>MILVNKETRVLVQGITGREGQFHTKQMLSYGTKIVAGVTPGKGGMEVLGVPVYDTVKEAVAHHEVDASIIFVPAPAAADAALEAAHAGIPLIVLITEGIPTLDMVRAVEEIKALGSRLIGGNCPGIISAEETKIGIMPGHVFKRGRVGIISRSGTLTYEAAAALSQAGLGTTTTVGIGGDPVIGTTFKDLLPLFNEDPETEAVVLIGEIGGSDEEEAAAWVKDHMKKPVVGFIGGRSAPKGKRMGHAGAIIMGNVGTPESKLRAFAEAGIPVADTIDEIVELVKKALGWNSRPGIL[4x];>[4x]MNLHEYQAKEILARYGVPVPPGKVAYTPEEAKRIAEEFGKRVVIKAQVHVGGRGKAGGVKLADTPQEAYEKAQAILGMNIKGLTVKKVLVAEAVDIAKEYYAGLILDRAKKRVVLMLSKEGGVDIEEVAAERPEAIHKFWIDPHKGFRPFEAREMVKRAGLEGNLNKLAQVLVALYRAYEGVDASIAEINPLVVTTDGGIVAADAKIVLDDNALFRHPDLAELREVEAEHPLEVEASNYGFAYVKLDGNIGIIGNGAGLVMYTLDLVNRVGGKPANFLDIGGGAKADVVYNALKVVLKDPDVKGVFINIFG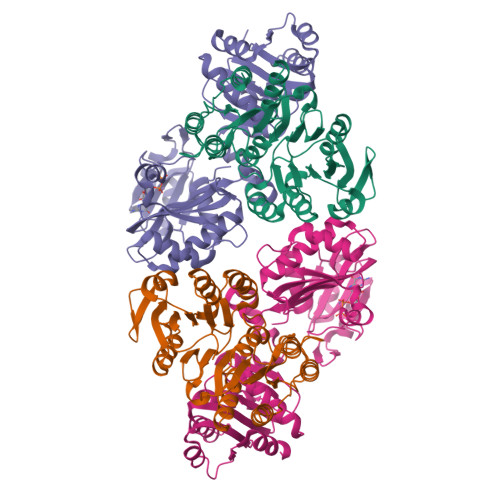GITRADEVAKGVIRALEEGLLTKPVVMRVAGTAEEEAKKLLEGKPVYMYPTSIEAAKVTVAMKGGAAWLEFAPGDLPMVHSQYNLL> SNIQTGAERMPHDLSHLGFLAGQIGRLITISTTPVIAGDSFEMDAVGALRLSPLRRGLAIDSTVDIFTFYVPHRHVYGEQWIKFMKDGVNATPLPTVNTTGYIDHAAFLGTINPDTNKIPKHLFQGYLNIYNNYFKAPWMPDRTEANPNELNQDDARFGFRCCHLKNIWTAPLPPETELSRQMTTSTTSIDIMGLQAAYANLHTDQERD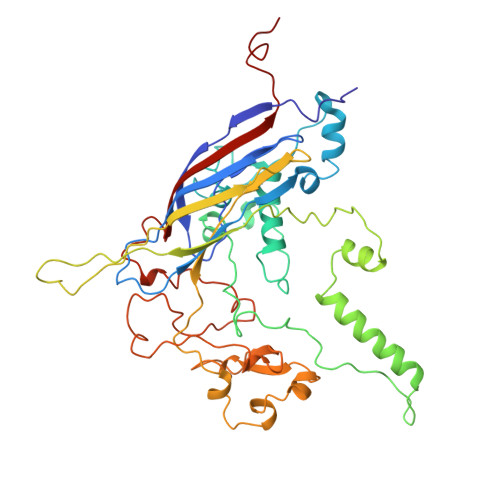YFMQRYRDVISSFGGKTSYDADNRPLLVMRSNLWASGYDVDGTDQTSLGQFSGRVQQTYKHSVPRFFVPEHGTMFTLALVRFPPTATKEIQYLNAKGALTYTDIAGDPVLYGNLPPREISMKDVFRSGDSSKKFKIAEGQWYRYAPSYVSPAYHLLEGFPFIQEPPSGDLQERVLIRHHDYDQCFQSVQLLQWNSQVKFNVTVYRNLPTTRDSIMTS>HMLRPVETPTREIKKLDGLWAFSLDRENCGIDQRWWESALQESRAIAVPGSFNDQFADADIRNYAGNVWYQREVFIPKGWAGQRIVLRFDAVTHYGKVWVNNQEVMEHQGGYTPFEADVTPYVIAGKSVRITVCVNNELNWQTIPPGMVITDENGKKKQSYFHDFFNYAGIHRSVMLYTTPNTWVDDITVVTHVAQDCNHASVDWQVVANGDVSVELRDADQQVVATGQGTSGTLQVV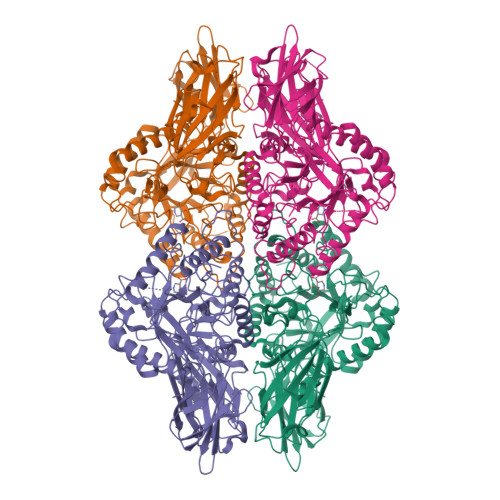NPHLWQPGEGYLYELCVTAKSQTECDIYPLRVGIRSVAVKGEQFLINHKPFYFTGFGRHEDADLRGKGFDNVLMVHDHALMDWIGANSYRTSHYPYAEEMLDWADEHGIVVIDETAAVGFNLSLGIGFEAGNKPKELYSEEAVNGETQQAHLQAIKELIARDKNHPSVVMWSIANEPDTRPQGAREYFAPLAEATRKLDPTRPITCVNVMFCDAHTDTISDLFDVLCLNRYYGWYVQSGDLETAEKVLEKELLAWQEKLHQPIIITEYGVDTLAGLHSMYTDMWSEEYQCAWLDMYHRVFDRVSAVVGEQVWNFADFATSQGILRVGGNKKGIFTRDRKPKSAAFLLQKRWTGMNFGEKPQQGGKQ[4x]> SLQRVPSYDSFDSEDYPAALPNHKPKGTFKDYVRDRADLNKDKPVIPAAALAGATGSGPIQ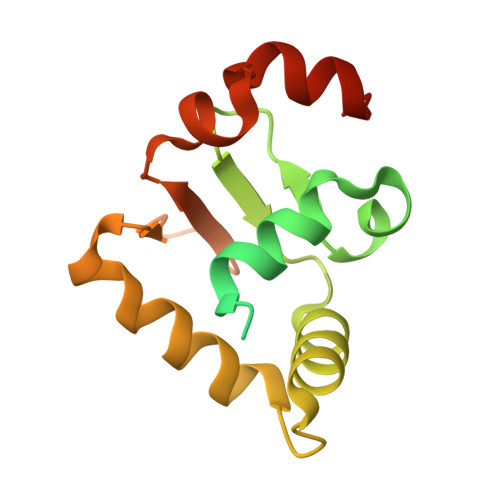LWQFLLELLTDKSCQSFISWTGDGWEFKLSDPDEVARRWGKRKNKPKMNYEKLSRGLRYYYDKNIIHKTAGKRYVYRFVCDLQSLLGYTPEELHAMLDVKPDADE> CC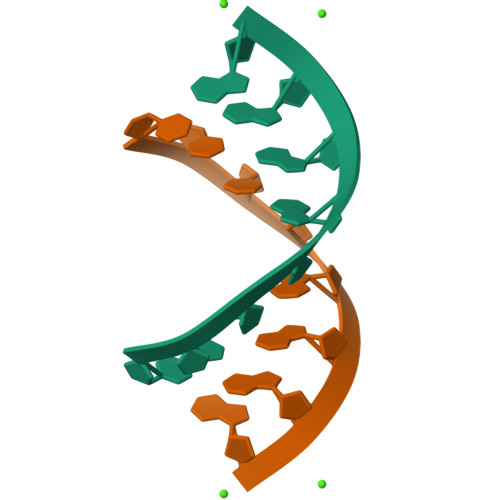CNGGGG> GEIEFIESSKDAGFPVINTPSKTKLEPSVFHQVFEGNKEPAVLRSGDPRLKANFEEAIFSKYIGNVNTHVDEYMLEAVDHYAGQLATLDISTEPMKLED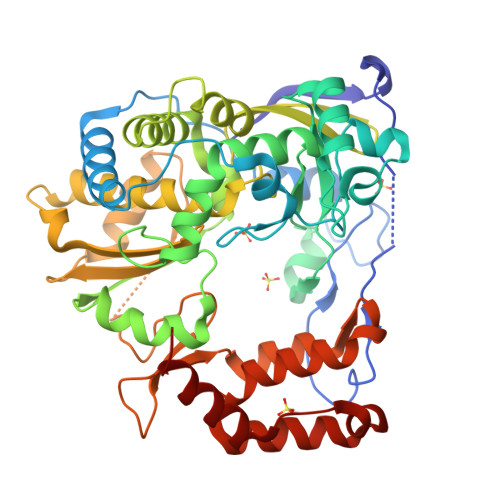AVYGTEGLEALDLTTSAGYPYVALGIKKRDILSKKTKDLTKLKECMDKYGLNLPMVTYVKDELRSIEKVAKGKSRLIEASSLNDSVAMRQTFGNLYKTFHLNPGVVTGSAVGCDPDLFWSKIPVMLDGHLIAFDYSGYDASLSPVWFACLKMILEKLGYTHKETNYIDYLCNSHHLYRDKHYFVRGGMPSGCSGTSIFNSMINNIIIRTLMLKVYKGIDLDQFRMIAYGDDVIASYPWPIDASLLAEAGKGYGLIMTPADKGECANEVTWTNVTFLKRYFRADEQYPFLVHPVMPMKDIHESIRWTKDPKNTQDHVRSLCLLAWHNGEHEYEEFIRKIRSVPVGRCLTLPAFSTLRRKWLDSFGSS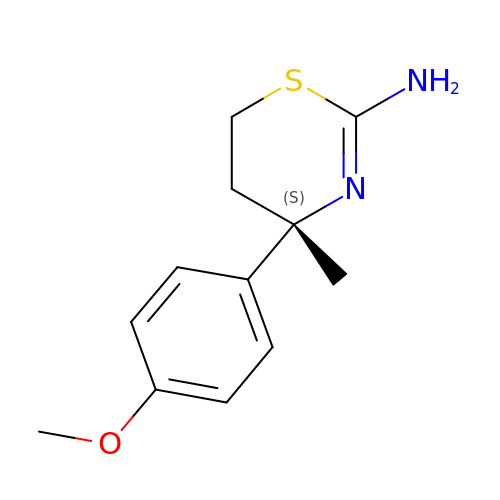(4S)-4-(4-methoxyphenyl)-4-methyl-5,6-dihydro-1,3-thiazin-2-amine | C12 H16 N2 O S | VKHSIJFRPDEMHV-LBPRGKRZSA-N>[4x]GFDYDGPLMKTEVPGPRSRELMKQLNIIQNAEAVHFFCNYEESRGNYLVDVDGNRMLDLYSQISSIPIGYSHPALVKLVQQPQNVSTFI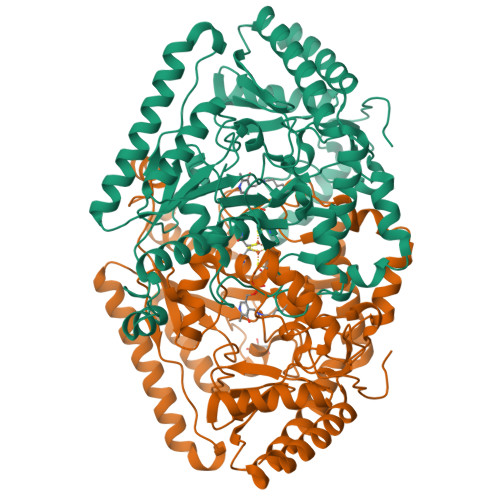NRPALGILPPENFVEKLRESLLSVAPKGMSQLITMACGSCSNENAFKTIFMWYRSKERGESAFSKEELETCMINQAPGCPDYSILSFMGAFHGRTMGCLATTHSKAIHKIDIPSFDWPIAPFPRLKYPLEEFVKENQQEEARCLEEVEDLIVKYRKKKKTVAGIIVEPIQSEGGDNHASDDFFRKLRDISRKHGCAFLVDEVQTGGGSTGKFWAHEHWGLDDPADVMTFSKKMMTGGFFHKEEFRPNAPYRIFNTWLGDPSKNLLLAEVINIIKREDLLSNAAHAGKVLLTGLLDLQARYPQFISRVRGRGTFCSFDTPDESIRNKLISIARNKGVMLGGCGDKSIRFRPTLVFRDHHAHLFLNIFSDILADFK> MN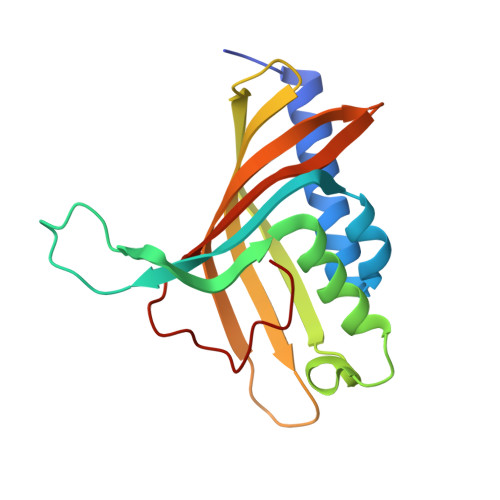TQTRVSDTTVREITEWLYMEAELLDAGKYREWLALVTEDLSYVVPIRVTREREAVTDVVEGMTHMDDDADSMEMRVLRLETEYAWAEDPPSRSRHFVTNVRVATGDSEDEFKVTSNLLLYRTRGDVATYDVLSGERTDVLRRAGDSFLMAKRVVLLDQTTIMTHNLALIM> SQSNRELVVDFLSYKLSQKGYSWSQMAAVKQALREAGDEFELRYRRAFSDLTSQLHITPGTAYQSFEQVVNELFRDGVNWGRIVAFFSFGGALCVESVDKEMQVLVSRIAAWMATYLNDHLE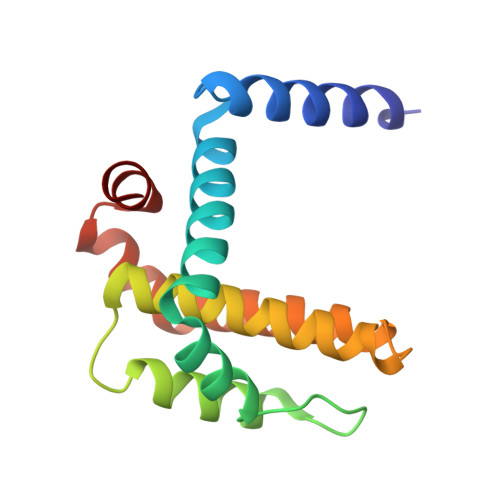PWIQENGGWDTFVELY> GSASAQSRTLAGGIHATDLNDKSVQRALDFAISEYNKVINKDEYYSRPLQVMAAYQQIVGGVNYYFNVKFGRTTCTKSQPNLDNCPFNDQPKLKEEEFCSFQINEVPWEDKI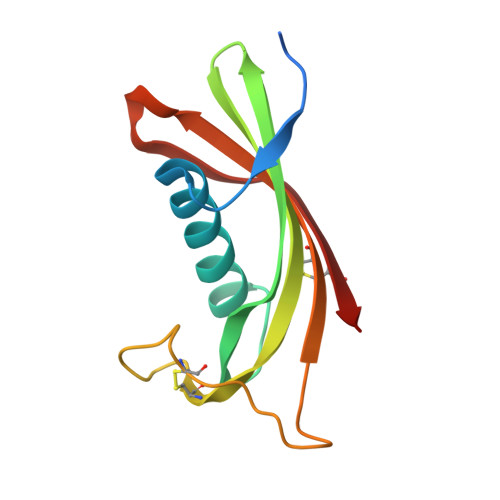SILNYKCRKV> ATSDSNMLLNYVPVYVMLPLGVVNVDNVFEDPDGLKEQLLQLRAAGVDGVMVDVWWGIIEL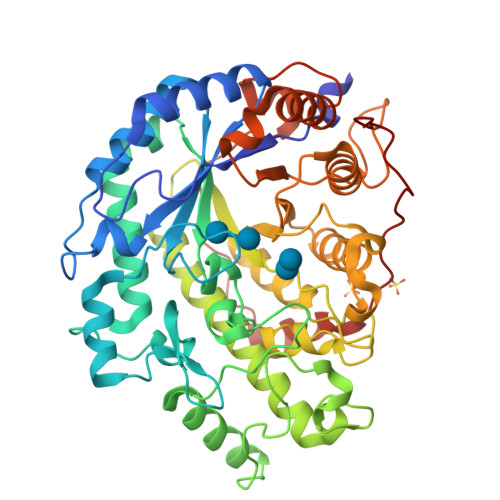KGPKQYDWRAYRSLLQLVQECGLTLQAIMSFHQCGGNVGDIVNIPIPQWVLDIGESNHDIFYTNRSGTRNKEYLTVGVDNEPIFHGRTAIEIYSDYMKSFRENMSDFLESGLIIDIYVGLGPAGELRYPSYPQSQGWEFPGIGEFQCYDKYLKADFKAAVARAGHPEWELPDDAGKYNDVPESTGFFKSNGTYVTEKGKFFLTWYSNKLLNHGDQILDEANKAFLGCKVKLAIKVSGIHWWYKVENHAAELTAGYYNLNDRDGYRPIARMLSRHHAILNFTCLEMRDSEQPSDAKSGPQELVQQVLSGGWREDIRVAGENALPRYDATAYNQIILNARPQGVNNNGPPKLSMFGVTYLRLSDDLLQKSNFNIFKKFVLKMHADQDYCANPQKYNHAITPLKPSAPKIPIEVLLEATKPTLPFPWLPETDMKVDG>QTPDKAKEQHPKLETYRCTKASGCKKQTNYIVADAGIHGIRQKNGAGCGDWGQKPNATACPDEASCAKNCILSGMDSNAYKNAGITTSGNKLRLQQLINNQLVSPRVYLLEENKKKYEMLHLTGTEFSFDVEMEKLPCGMNGALYLSEMPQDGGKSTSRNSKAGAYYGAGYCDAQCYVTPFINGVGNIKGQGVCCNELDIWEANSRATHIAPHPCSKPGLYGCTGDECGSSGICDKAGCGWNHNRINVTDFYGRGKQYKVDSTRKFTVTSQFVANKQGDLIELHRHYIQDNKV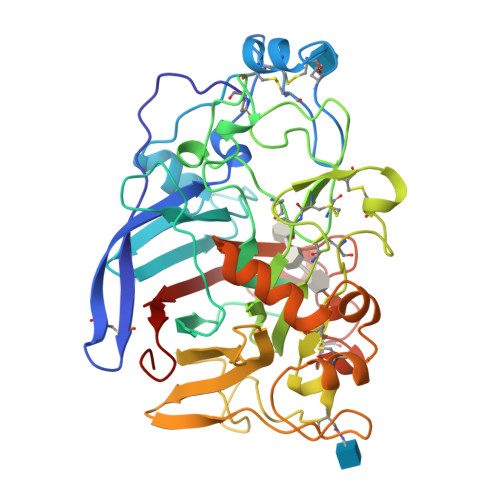IESAVVNISGPPKINFINDKYCAATGANEYMRLGGTKQMGDAMSRGMVLAMSVWWSEGDFMAWLDQGVAGPCDATEGDPKNIVKVQPNPEVTFSNIRIGEIGSTS[4x]(3S)-3-(5,5-dimethyl-2-oxo-1,3-oxazolidin-3-yl)-N-(1H-tetrazol-5-yl)-1-[3-(trifluoromethyl)benzoyl]-2,3-dihydro-1H-indole-3-carboxamide 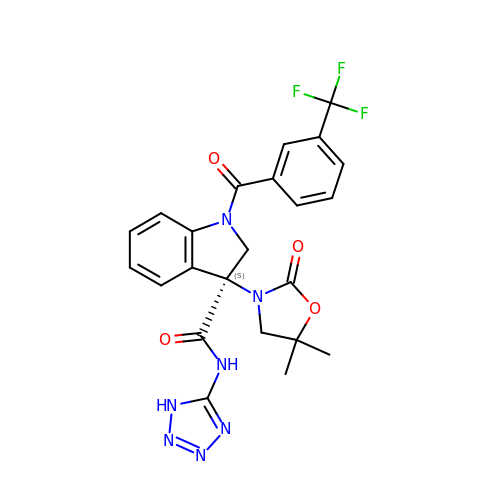| C23 H20 F3 N7 O4 | CIOWYUCMYWZPAD-JOCHJYFZSA-N> MDFFNKFSQGLAESSTPKSSIYYSEEKDPDTKKDEAIEIGLKSQESYYQRQLREQLARDNMTVASRQPIQPLQPTIHITPQPVPTATPAPILLPSSTVPTPKPRQQTNTSSDMSNLFDWLSEDTDAPASSLLPALTPSNAVQDIISKFNKDQKTTTPPSTQPSQTLPTTTCTQQ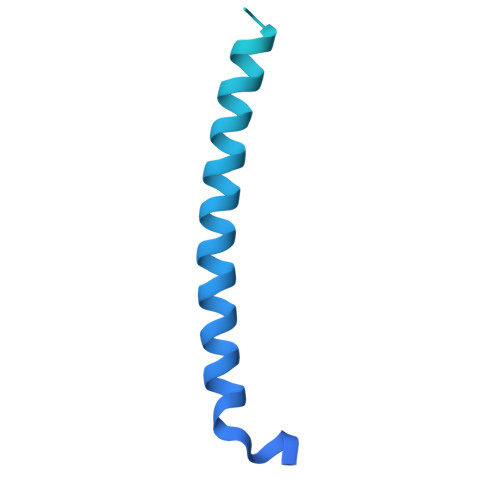SDGNISCTTPTVTPPQPPIVATVCTPTPTGGTVCTTAQQNPNPGAASQQNLDDMALKDLMSNVERDMHQLQAETNDLVTNVYDAREYTRRAIDQILQLVKGFERFQK>[4x]GSAAAESGTISNNWSIEQHPNYYHVEGKAQLDIKNFPELYRTTERVYKKSGQSTKPVTVSNIHYSVLDGYGRSGEAYGIITKDMIDMSAGYREKWESK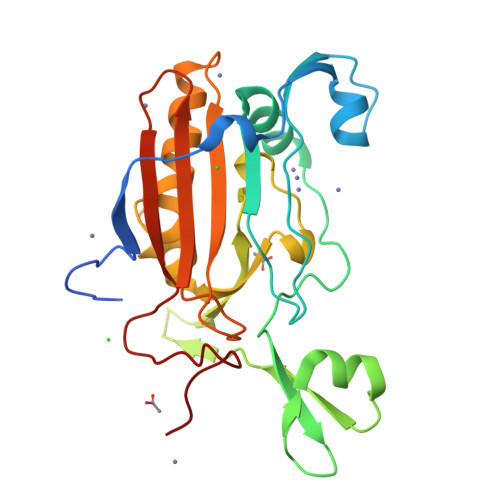PEPSGWYSYFFKNTNQRATESDYKHSPKNVSKISNNIKASILLSNGNVRNGYLFDRSGLIADSLGGRPFRNNLITGTRTQNVGNNDRKGGMQYIENKVLDHIKRNPKVHVYYKATPVYQGSELLPRAVLVSALSSDGFIDETVRVFNNVAGFNIDYQNGGLLSS> QVNRLPFFTNHFFDTYLLISEDTPVGSSVTQLLARDMDNDPLVFGVSGEEASRFFAVEPDTGVVWLRQPLDRETKSEFTVEFSVSDHQGVITRKVNI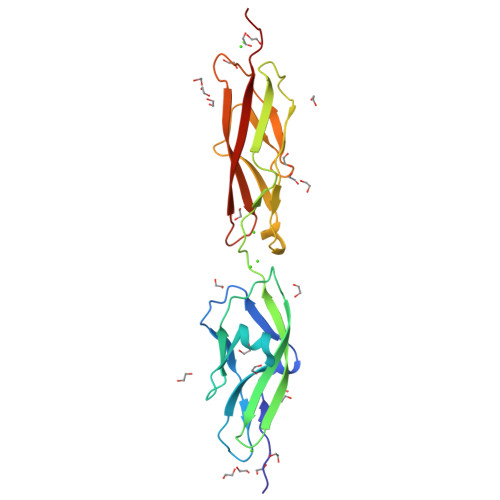QVGDVNDNAPTFHNQPYSVRIPENTPVGTPIFIVNATDPDLGAGGSVLYSFQPPSPFFAIDSARGIVTVIQELDYEVTQAYQLTVNATDQDKTRPLSTLANLAIIITDMQDMD>MPSNMKQFCKISVWLQQHDPDLLEIINNLCMLGNLSAAKYKHGVTFIYPKQAKIRDEIKKHAYSNDPSQAIKTLESLILPFYIPTPAEFTGEIGSYTGVKLEVEKTEANKVILKNGEAVLVPAADFKPFPDRRLAVWIMESGSMPLEGPPYKRKK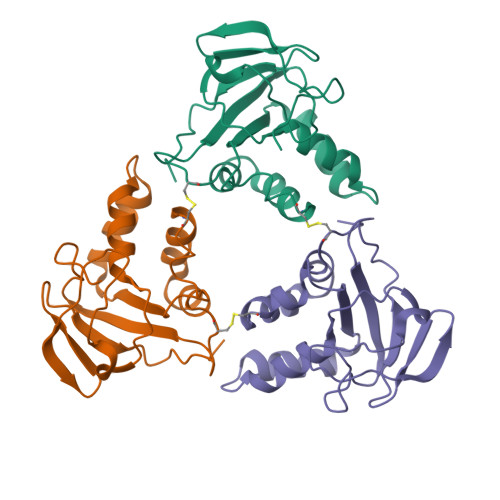EGGGNLEHHHHHHHH[3x]> VPAPGETRACGRKLISLVMAVCGDLCNPQEGKDIAT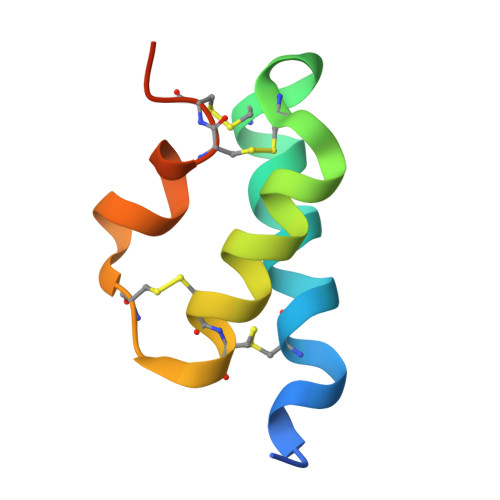ECCGNQCSDDYIRSACCPHHHHHH>[28x]MPPRPLDVLNRSLKSPVIVRLKGGREFRGTLDGYDIHMNLVL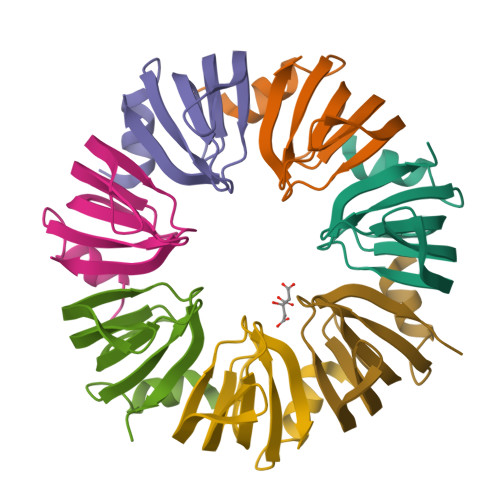LDAEEIQNGEVVRKVGSVVIRGDTVVFVSPAPGGE1-VINYLIMIDAZOLE | C5 H7 N2 | 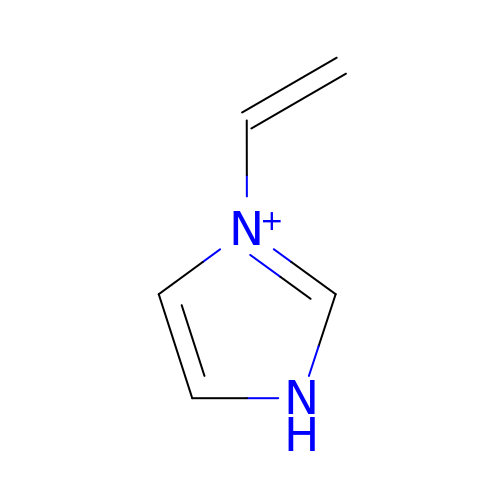OSSNTDFYBPYIEC-UHFFFAOYSA-O>GSMGNLAEKMYKAGNAMYRKGQYTIAIIAYTLALLKDPNNAEAWYNLGNAAYKKGEYDEAIEAYQKALELDPNNAEAWYNLGNAYYKQGDYDEAIEYYKKALRLDPRNVDAIENLIEAEEKQGAS[12x];>MEEAELAYLLGELAYKLGEYRIAIRAYRIALKRDPNNAEAWYNLGNAYYKQGDYREAIRYYLRALKLDPENAEAWYNLGNALYKQGKYD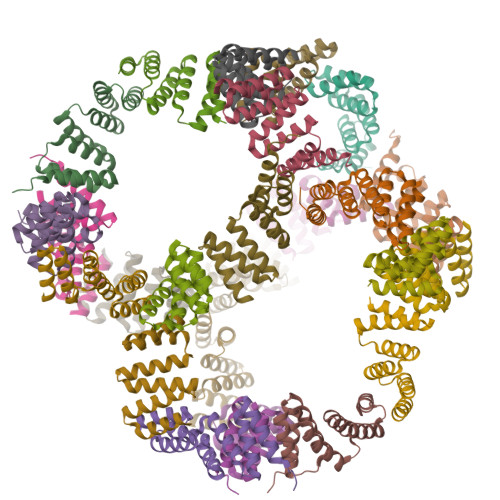LAIIAYQAALEEDPNNAEAKQNLGNAKQKQGLEHHHHHH[12x]> AITGIFFGSDTGNTENIAKMIQKQLGKDVADVHDIAKSSKEDLEAYDILLLGIPTWYYGEAQCDWDDFFPTLEEIDFNGKLVALFGCGDQEDYAEYFCDALGTIRDIIEPRGATIVGHWPTAGYHFEASKGLADDDHFVGLAIDEDRQPELT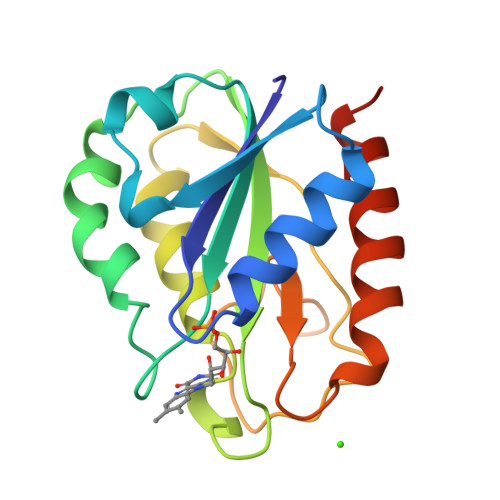AERVEKWVKQISEELHLDEILNA>[2x]GSHMAKEEIIWESLSVDVGSQGNPGIVEYKGVDTKTGEVLFEREPIPIGTNNMGEFLAIVHGLRY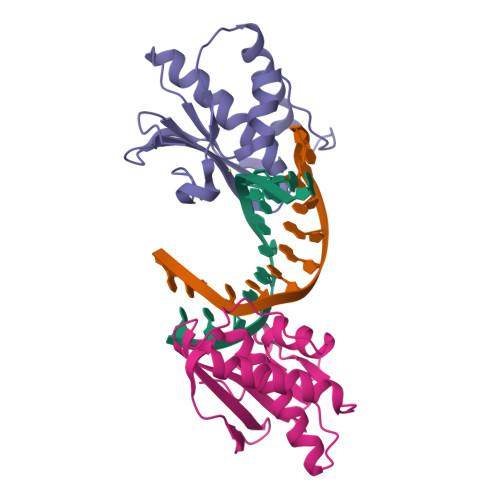LKERNSRKPIYSDSQTAIKWVKDKKAKSTLVRNEETALIWKLVDEAEEWLNTHTYETPILKWQTDKWGEIKANY> IPTNLRVLR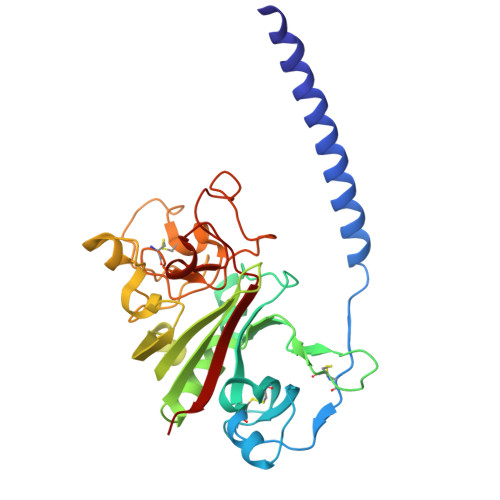SILENLRSKIQKLESDVSAQMEYCRTPCTVSCNIPVVSGKECEEIIRKGGETSEMYLIQPDSSVKPYRVYCDMNTENGGWTVIQNRQDGSVDFGRKWDPYKQGFGNVATNTDGKNYCGLPGEYWLGNDKISQLTRMGPTELLIEMEDWKGDKVKAHYGGFTVQNEANKYQISVNKYRGTAGNALMDGASQLMGENRTMTIHNGMFFSTYDRDNDGWLTSDPRKQCSKEDGGGWWYNRCHAANPNGRYYWGGQYTWDMAKHGTDDGVVWMNWKGSWYSMRKMSMKIRPFF>QVTVIPREQHAISRKDISENALKVMYRLNKAGYEAWLVGGGVRDLLLGKKPKDFDVTTNATPEQVRKLFRNCRLVGRRFRLAHVMFGPEIIEVATFRGHHEGNVSDRTTSQRGQNGMLLRDNIFGSIEEDAQRRDFTINSLYYSVADFTVRDYVGGMKDLKDGVIRLIGNPETRYREDPVRMLRAVRFAAKLGMRISPETAEPIPRLATL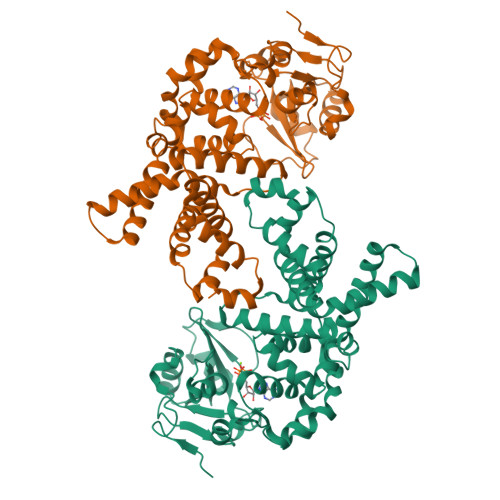LNDIPPAHLFEESLKLLQAGYGYETYKLLCEYHLFQPLFPTITRYFTENGDSPMERIIEQVLKNTDTRIHNDMRVNPAFLFAAMFWYPLLETAQKIAQESGLTYHDAFALAMNDVLDEACRSLAIPKRLTTLTRDIWQLQLRMSRRQGKRAWKLLEHPKFRAAYDLLALRAEVERNAELQRLVKWWGEFQVSAPPDQKGMLNELD[2x]> HQLLSPSSFSPSATPSQKYNSRSNRGEVVTSFGLAQGVSWSGRGGAGNISLKVLGCPEALTGSYKSMFQKLPDIREVLTCKIEELGSELKEHYKIEAFTPLLAPAQEPVTLLGQIGCDSNGKLNNKSVILEGDREHSSGAQIPVDLSELKEYSLFPGQVVIMEGINTTGRKLVATKLYEGVPLPFYQPTEEDADFEQSMVLVACGPYTTSDSITYDPLLDLIAVINHDRPDVCILFGPFLDAKHEQVENCLLTSPFEDIFKQCLRTIIEGTRSSGSHLVFVPSLRDVHHEPVYPQPPFSYSDLSREDKKQVQFVSEPCSLSINGVIFGLTSTDLLFHLGAEEISSSSGTSDRFSRILKHILTQRSYYPLYPPQEDMAIDYESFYVYAQLPVTPDVLIIPSELRYFVKDVLGCVCVNPG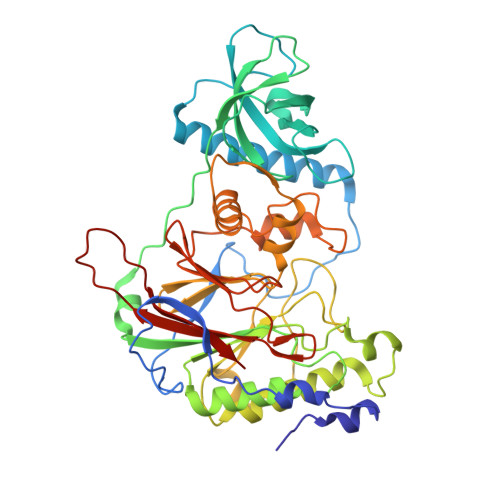RLTKGQVGGTFARLYLRRPAADGAERQSPCIAVQVVRI>MTAPRSWAPTTRARGDTEALCSPEDGWVKVHPTPGTMLFREILHGQLGYTEGQGVYNVVRSSEATTRQLQAAIFHALLNATTYRDLEADWLGHVAARGLQPQRLVRRYRNAREADIAGVAERVFDTWRNTLRTTLLDFAHGLVACFAPGGPSGPSSFPKYIDWLTCLGLVPILRKRQEGGVTQGLRAFLKQHPLTRQLATVAEAAERAGPGFFELALAFDSTRVADYDRVYIYYNHRRGDWLVRDPISGQRGECLVLWPPLWTGDRLVFDSPVQRLFPEIVACHSLREHAHVCRLRNTASVKVLLGRKSDSERGVAGAARVVNKVLGEDDETKAGSAASRLVRLIINMKGMRHVGDINDTVRAYLDEAGGHLIDAPAVDGTLPGFGKGGNSRGSAGQDQGGRAPQLRQAFRTAVVNNINGVLEGYINNLFGTIERLRETNAGLATQLQERDRELRRATAGALERQQRAADLAAESVTGGCGSRPAGADLLRADYDIIDVSKSMDDDTYVANSFQHPYIPSYAQDLERLSRLWEHELVRCFKILCHRNNQGQETSISYSSGAIAAFVAPYFESVLRAPRVGAPITGSDVILGEEELWDAVFKKTRLQTYLTDIAALFVADVQHAALPPPPSPVGADFRPGASPRGRSRSRSPGRTAPGAPDQGGGIGHRDGRRDGRR[12x]

Three capsid types have been recognized from the nuclei of herpesvirus-infected cells: empty A-capsids, scaffolding-containing B-capsids, and DNA-filled C-capsids. A unique portal vertex exists at a 12th I5 vertex through which the genome is translocated during assembly. Here, portal proteins assemble into a dodecameric basket-like structure that is thought to seed the assembly of scaffolding proteins, in turn driving the formation of spherical procapsids composed of MCP, SCP, and triplexes. A separate protein complex, the terminase, associates with the dodecameric portal and initiates genome packaging and the concurrent autoproteolytic cleavage of the scaffold.

The resultant atomic structures reveal not only the expected A-, B-, and C-capsids but also capsids with portal vertices similar to C-capsids but no resolvable genome in the capsid lumen, which we named D-capsids. In addition to features consistent with previous herpesvirus structures, our data set reveals a previously unidentified capsid end product. These new capsids feature C-capsid-like “elevated” portals and, in many cases, terminal genome within the portal translocation channel, but no organized genome in the capsid lumen. We refer to these capsids as “D-capsids” because their C-capsid-like portal suggests they were originally C-capsids, but the absence of most of the genome indicates that they are degraded. In D-capsids, terminal DNA density exists in multiple conformations including one reminiscent of that in C-capsids, suggesting D-capsids are products of failed DNA retention. However, our D-capsid portal structures have the same portal basket position as C-capsids despite being mostly devoid of genome. These observations together suggest that genome pressure alone does not determine portal basket height, and the elevated portal position observed in C- and D-capsids may instead be an irreversible step during capsid maturation. D-capsid portals had 4 Å variability in height, but otherwise resembled C-capsid portals. The C12 reconstruction of both A- and B-capsid portal baskets revealed a small hook-like density with large aromatic side chains and sharp turns wedged into a hydrophobic pocket between the crown domains of each portal monomer. This density is weaker in A-capsids, but still conspicuous, whereas it is completely absent in C-capsids, D-capsids, and mature virions (Fig. 4C through E and H through J).>[2x]GPGSMYRSRPEPVQGHLFTYYKDPYCKIPVFMMNMDARRCVLWVGGQTESLLSFDYFTNLAEELQGDWAFVQVEVPSGKIGSGPQDHAHD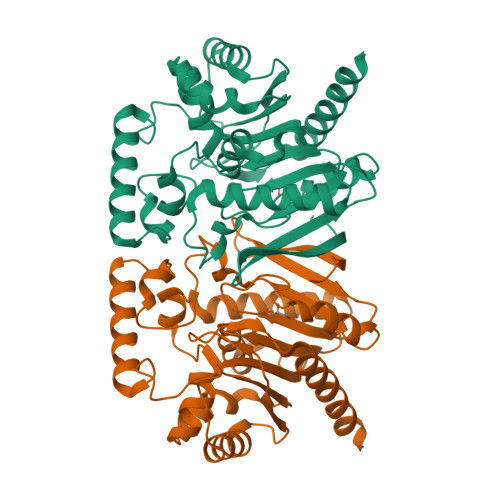AEDVDDLIGILLRDHCMNEVALFATSTGTQLVFELLENSAHKSSITRVILHGVVCDPENPLFTPEGCAARKEHVEKLMAEGRGEDSLAMLKHYDIPITPARLAGGGFPTLQEAVWNPCIRKEFDVLRRSVGVIKVPLLLMLAHNVQYKPSDEEVGTVLEGVRDHTGCNRVTVSYFNDTCDELRRVLKAAESEHVAAILQFLADEDEFRTETEKNNRIKAAEDEKKRKSVLQVSSFAQAASSVKAS Natural competence is the term used to describe the uptake of “naked” extracellular DNA by bacteria; it plays a significant role in horizontal genetic exchange. Previous work on T. thermophilus HB27 by Friedrich et al. identified a locus containing five open reading frames (ORFs) associated with natural competence. Four ORFs (pilA1 to pilA4 [pilA1-4]) were type IVa pilin-like genes, and a fifth, comZ, encoded an unusual and much larger protein that lacked some of the sequence features characteristic of pilin genes. Mutation of pilA1-3 and comZ leads to a loss of natural competence, although piliation is maintained.

Three competence-associated pilin genes, pilA1-pilA2-pilA3, are found adjacent to comZ in the T. thermophilus strain HB27 genome. Unlike ComZ, each ORF was positively identified as a type IV pilin by PilFind. PilA2 gave crystals with good diffraction qualities, and the structure was determined to 1.39-Å resolution; it forms a distinctly identifiable domain with a small subdomain insertion. PilA2 adopts a type IV pilin fold, a single α-helix packed against four antiparallel β-strands, with a small subdomain inserted between the end of the first α-helix and the beginning of the fourth β-strand, consisting of three short antiparallel β-strands and a short α-helix, linked by an extensive loop region. A search with DALI identified close structural homology with the type II secretion system pseudopilins EpsI from Vibrio vulnificus and GspI from E. coli, as well as the minor type IV pilin TTHA1218 from T. thermophilus HB8 (35). Although all three related pilin structures share the same fold, the subdomain is consistently absent. ComZ binds specifically to the competence-associated pilin PilA2. The ComZ/PilA2 complex eluted in a single peak (∼80 kDa), at a higher apparent mass than ComZ alone (∼60 kDa); the complex peak contained both proteins (lower). Specific binding of the two proteins was confirmed by isothermal titration calorimetry (ITC), which gave a stoichiometry of 1.1 and an equilibrium binding constant (Kd) of 0.69 μM. Our model for the ComZ/PilA2 complex underscores this point by locating PilA2 such that its smaller subdomain sits between the ComZ pilin and β-solenoid domains, suggesting that ComZ could effectively cap the end of the competence pilus fiber. Virtually no reduction in DNA mobility was recorded in the presence of PilA2 alone.

>NLRASAQARFATDAKAAAVQVLERRSAEVLKSEIVPALSPYKDAPLDPDNPSGNWRSFYFVDYYFSCPTRVAPSPKQRGGSVANLRPGLTCSGTETIFGIPVAWDIRGENGILGEGVVTVVVTATHPRGPKVTLGRRVTCYDVYPSPTQDQPAPCPPPGGGRPGSGSWSHPQFEK[4x]beta-L-psicofuranose | C6 H12 O6 | 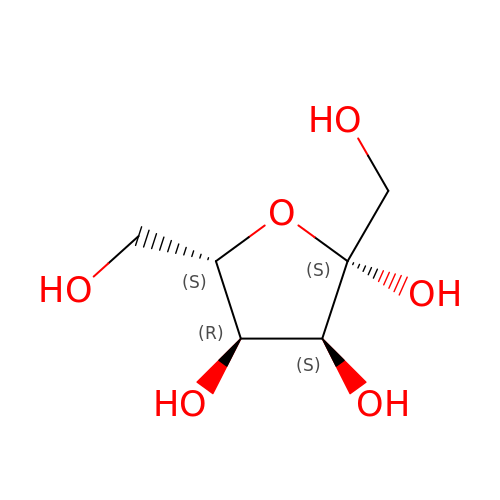RFSUNEUAIZKAJO-BXKVDMCESA-N>GSHMRSRRVDVMDVMNRLILAMDLMNRDDALRVTGEVREY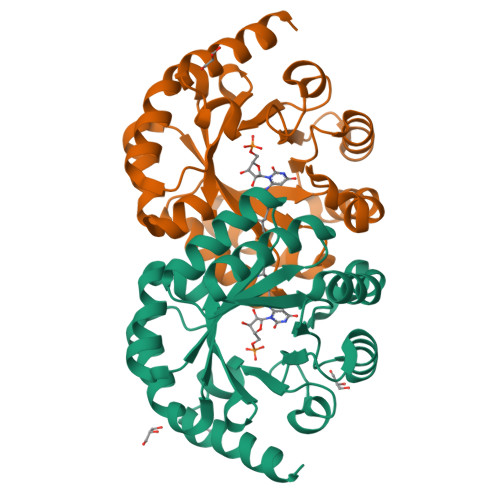IDTVKIGYPLVLSEGMDIIAEFRKRFGCRIIADFKVADIPETNEKICRATFKAGADAIIVHGFPGADSVRACLNVAEEMGREVFLLTEMSHPGAEMFIQGAADEIARMGVDLGVKNYVGPSTRPERLSRLREIIGQDSFLISPGVGAQGGDPGETLRFADAIIVGRSIYLADNPAAAAAGIIESIKDLRIPEDPAANKARKEAELAAATAEQ[2x]> GIEDLIDTAIKNALRVSQPPSTQSTEATSGVNSQEVPALTAVETGASGQAIPSDVVETRHVVNYKTRSESCLESFFGRAACVTILSLTNSSKSGEEKKHFNIWNITYTDTVQLRRKLEFFTYSRFDLEMTFVFTENYPSTASGEVRNQVYQIMYIPPGAPRPSSWDDYTWQSSSNPSIFYMYGNAPPRMSIPYVGIANAYSHFYDGFARVPLEGENTDAGDTFYGLVSINDFGV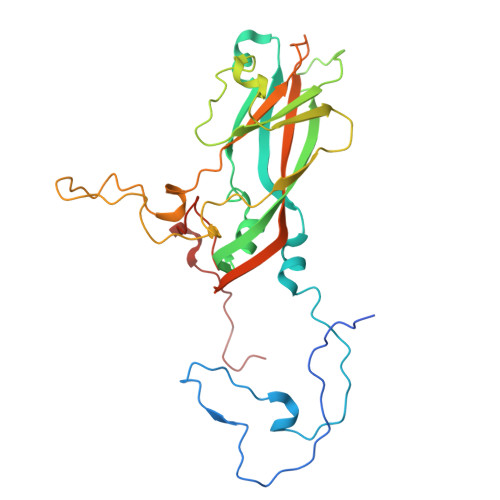LAVRAVNRSNPHTIHTSVRVYMKPKHIRCWCPRPPRAVLYRGEGVDMISSAILPLAKVDSITTF We previously identified EilR as a regulatory component of a multidrug efflux system from Enterobacter lignolyticus, a bacterium isolated from the soil of a Puerto Rican rainforest because of its ability to catabolize lignin components. In its native context, EilR regulates expression of EilA, an inner membrane transporter that confers tolerance to imidazolium-based ionic liquids, reagents that enhance the microbial conversion of lignocellulosic biomass to chemicals. EilR belongs to the TetR family of transcription factors, which commonly regulate divergently transcribed adjacent genes. Amino acid residues 1–192 of each monomer form 9 α-helices arranged in two domains: the N-terminal DNA-binding domain consists of residues 1–52, forming three α-helices, and the C-terminal ligand-binding domain comprises residues 53–192, forming six α-helices.

In a similar manner to the EilR-operator complex, we used crystallography to investigate the EilR structure in complex with each of two cationic triarylmethane ligands, malachite green (MG) and the most potent inducer CV. Structural analysis revealed the binding of two ligand molecules per EilR dimer. The ligand-binding site of EilR contains several Glu and Asp residues, a distinctive feature this repressor shares with other transcription factors that recognize small cationic molecules. To demonstrate the specificity of these negatively charged residues for ligand binding, we created Ala substitutions of EilR and examined their ability to de-repress RFP expression via PJExD in the presence of MG and CV. While the Glu90 and Asp175 mutants induced RFP to a similar extent as wild-type EilR, the absence of Asp163 caused a dramatic decrease in expression, suggesting that Asp163 is required for EilR to recognize the positive charge of these inducers. While several of the EilR-inducing dyes, notably methylene blue and malachite green, inhibited growth of E. coli at high concentrations, CV, acridine orange, and pyronin had only minimal effects on growth rate at concentrations required for full induction. Comparison of EilR in its induced and DNA-bound forms showed a significant conformational change around the ligand-binding sites.

>MGYLNREERRETIMQAAMRVALDQGFTGMTVRNIATAAGVAAGQVHHHFTSSGELKSQAFIRVIREMMDLQRLSRTAGWREQLFSALGSEDGRLEPYIRLWRQAQLLADSDPEIKSAYLLTMNLWHDEAVRIIRAGHAAGEFTLRDSAENIAWRLISLVCGLDGIYVLGMPEVDDAAFTRHLQHVIQLELFS[8x]>GMTSLPLEANAAATLAEWHGLIARRDLSGLPRLLHPDAVFRSPMAHKPYAGAPVVSMILNTVLTVFEDFAYHRQLASADGRSVVLEFSARVGERELKGIDMIRFDDDGRIVDFEVMVRPMSGLQALGEEMGRRLASY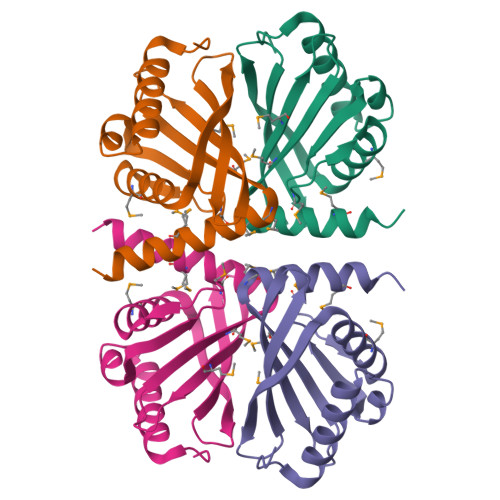LAASKA[2x]> MQPVYPEVKPNPLRNANLCSRIFFWWLNPLFKIGHKRRLEEDDMYSVLPEDRSQHLGEELQGYWDQEVLRAEKDAREPSLTKAIIKCYWKSYVVLGIFTLIEESTRVVQPIILGKIIGYFENYDPSDSAALYEAHGYAGVLSACTLVLAILHHLYFYHVQCAGMRLRVAMCHMIYRKALRLSNSAMGKTTTGQIVNLLSNDVNKFDQ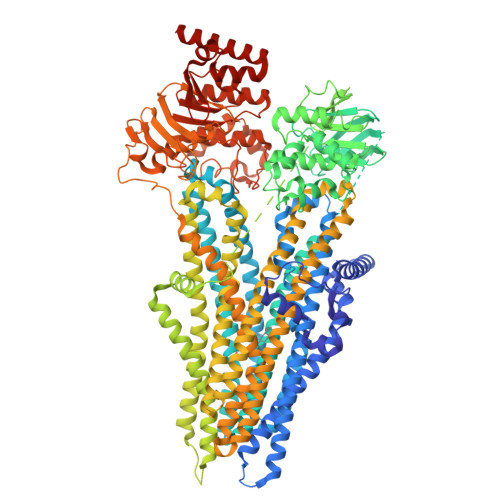VTIFLHFLWAGPLQAIVVTALLWMEIGISCLAGMAVLIILLPLQSCIGKLFSSLRSKTAAFTDTRIRTMNEVITGIRIIKMYAWEKSFADLITNLRRKEISKILRSSYLRGMNLASFFVASKIIVFVTFTTYVFLGNVITASRVFVAVSLYGAVRLTVTLFFPSAVEKVSEAFVSIRRIKNFLLLDEITQLHSQLPSDGKMIVNVQDFTAFWDKASDTPTLQSLSFTVRPGELLAVVGPVGAGKSSLLSAVLGELPPNQGQVSVHGRIAYVSQQPWVFSGTVRSNILFGKKYEKERYEKVIKACALKKDLQLLEDGDLTMIGDRGTTLSGGQKARVNLARAVYQDADIYLLDDPLSAVDAEVSRHLFELCICQALHEKIRILVTHQLQYLKAASQILILKDGQMVQKGTYTEFLKSGIDFGSLLKKENEEAEPSPVPGSPTLRNRTFSESSVWSQQSSRPSLKEATPEGQDTENIQVTLTEESRSEGKVGFKAYKNYFTAGAHWFIIIFLILVNLAAQVSYILQDWWLSYWANQQSALNVTVNGQGNVTEKLDLNWYLGIYSGLTASTVLFGIVRSLLVFFVLVSSSQTLHNQMFESILRAPVLFFDRNPIGRILNRFSKDIGHMDDLLPLTYLDFIQTFLQVIGVVGVAVAVIPWIAIPLVPLGIVFFVLRRYFLETSRDVKRLESTTRSPVFSHLSSSLQGLWTIRAYKAEQRFQELFDSHQDLHSEAWFLFLTTSRWFAVRLDAICAVFVIVVAFGSLILAKTLDAGQVGLALSYALTLMGMFQWCVRQSAEVENMMISVERVIEYTDLEKEAPWEYQKRPLPSWPHEGVIIFDNVNFSYSLDGPLVLKHLTALIKSKEKVGIVGRTGAGKSSLIAALFRLSEPEGKIWIDKILTTEIGLHDLRKKMSIIPQEPVLFTGTMRKNLDPFNEHSDEELWNALEEVQLKEAIEDLPGKMDTELAESGSNFSVGQRQLVCLARAILRKNRILIIDEATANVDPRTDELIQKKIREKFAHCTVLTIAHRLNTIIDSDKIMVLDSGRLKEYDEPYVLLQNRDSLFYKMVQQLGKAEAAALTETAKQVYFKRNYPDITHNGHVVMNASSGQPSAFTIFETAL>LKVREDENNPFYFRSSNSFQTLFENQNGRIRLLQRFNKRSPQLENLRDYRIVQFQSKPNTILLPHHADADFLLFVLSGRAILTLVNNDDRDSYNLHPGDAQRIPAGTTYYLVNPHDHQNLKIIKLAIPVNKPGRYDDFFLSSTQAQQSYLQGFSHNILETSFHSEFEEINRVLFGEEEEQRQQEGVIVELSKEQIRQLSRRAKSSSRKTISSEDEPFNLRSRNPIYSNNFGKFFEITPEKNPQLRDLDIFLSSVDINEGALLLPHFNSKAIVILVINEGDANIELVGIKEQQQKQKQEEE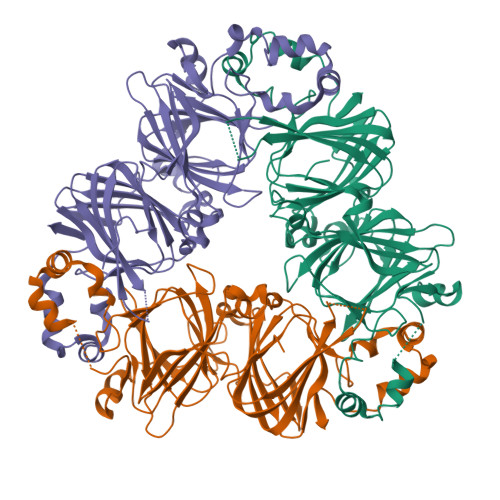PLEVQRYRAELSEDDVFVIPAAYPFVVNATSNLNFLAFGINAENNQRNFLAGEKDNVVRQIERQVQELAFPGSAQDVERLLKKQRESYFVDAQPQQKEEGSKGRKGPFPSILGALY[3x]> TTVPDLESDSFHVDWYRTYAELRETAPVTPVRFLGQDAWLVTGYDEAKAALSDLRLSSDPKKKYPGVEVEFPAYLGFPEDVRNYFATNMGTSDPPTHTRLRKLVSQEFTVRRVEAMRPRVEQITAELLDEVGDSGVVDIVDRFAHPLPIKVICELLGVDEKYRGEFGRWSSEILVMDPERAEQRGQAAREVVNFILDLVERRRTEPGDDLLSALIRVQDDDDGRLSADELTSIALVLLLAGFESSVSLIGIGTYLLLTHPDQLALVRRDPSALPNAVEEILRYIAPPETTTRFAA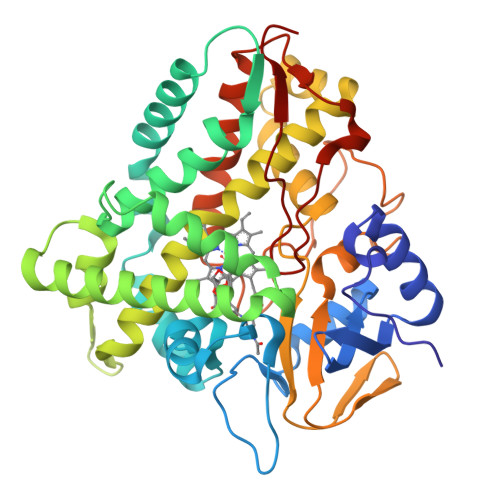EEVEIGGVAIPQYSTVLVANGAANRDPKQFPDPHRFDVTRDTRGHLSFGQGIHFCMGRPLAKLEGEVALRALFGRFPALSLGIDADDVVWRRSLLLRGIDHLPVRLDG> MEAALLVCQ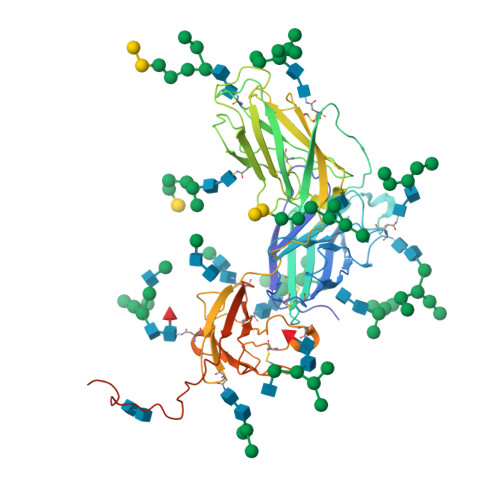YTIQSLIQLTRDDPGFFNVEILEFPFYPACNVCTADVNATINFDVGGKKHKLNLDFGLLTPHTKAVYQPRGAFGGSENATNLFLLELLGAGELALTMRSKKLPINITAGEEQQVSLESVDVYFQDVFGTMWCHHAEMQNPVYLIPETVPYIKWDNCNSTNITAVVRAQGLDVTLPLSLPTSAQDSNFSVKTEMLGNEIDIECIMEDGEISQVLPGDNKFNITCSGYESHVPSGGILTSTSPVATPIPGTGYAYSLRLTPRPVSRFLGNNSILYVFYSGNGPKASGGDYCIQSNIVFSDEIPASQDMPTNTTDITYVGDNATYSVPMVTSEDANSPNVTVTAFWAWPNNTETDFKCKWTLTSGTPSGCENISGAFASNRTFDITVSGLGTAPKTLIITRTATNATTTTHKVIFSKAPESTTTSPTLNTTGFAAPNTTTGLPSSTHVPTNLTAPTSTGPTVST> MPQLVPFYFMNQLTYGFLLMITLLILFSQF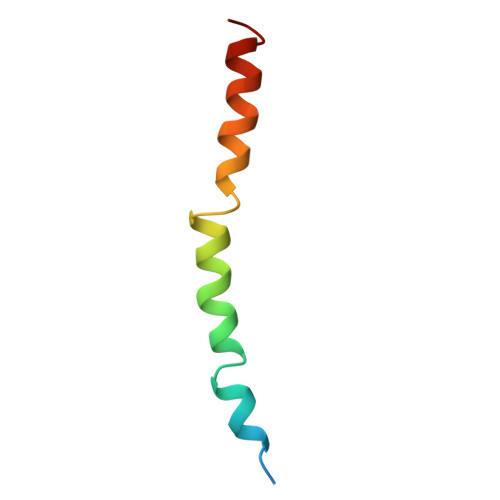FLPMILRLYVSRLFISKL>GHMTGAHERTFLAVKPDGVQRRLVGEIVRRFERKGFKLVALKLVQASEELLREHYAELRERPFYGRLVKYMASGPVVAMVWQGLDVVRTSRALIGATNPADAPPGTIRGDFCIEVGKNLIHGSDSVESARREIALWFRADELLCWEDSAGHWLYE[12x]

With regard to their common enzymatic activity, NDPKs are NTP/NDP transphosphorylases encoded by the nme genes. They catalyze the transfer of the γ-phosphate group from an NTP to an NDP via the formation of a high-energy intermediate on a catalytic histidine residue. We produced a truncated version of human NDPK isoform C (residues Thr18–Glu169, NDPK-C hereafter) and determined the 3D structure via X-ray crystallography in the absence and presence of various nucleotides. A data analysis revealed a hexameric arrangement, which is organized as three dimers, as previously reported for other functional eukaryotic NDPK variants.

In order to see differences in substrate recognition between adenosine and guanosine nucleotides, we crystallized NDPK-C in the presence of GDP, cAMP or UDP. Crystals with GDP belonged to space group P21, and the structure was solved at a resolution of 2.17 Å. For NDPK-C×GDP, we observed an unusual crystal packing: two hexamers contacted each other via Arg80 and GDP, sandwiching a SO42− ion from the crystallization screening solution. A further interaction between Asn112 (helix α2) of one hexamer and Pro76 of the neighboring hexamer could be observed. The residues contacting the guanine nucleotide base are the same as in the ADP complex, except for Glu169, which makes contact specifically with the guanine base in the adjacent protomer.> MGALRIDSHQHFWRYRAADYPWIGAGMGVLARDYLPDALHPLMHAQALGASIAVQARAGRDETAFLLELACDEARIAAVVGWEDLRAPQLAERVAEWRGTKLRGFRHQLQDEADVRAFVDDADFARGVAWLQANDYVYDVLVFERQLPDVQAFCARHDAHWLVLDHAGKPALAEFDRDDTAL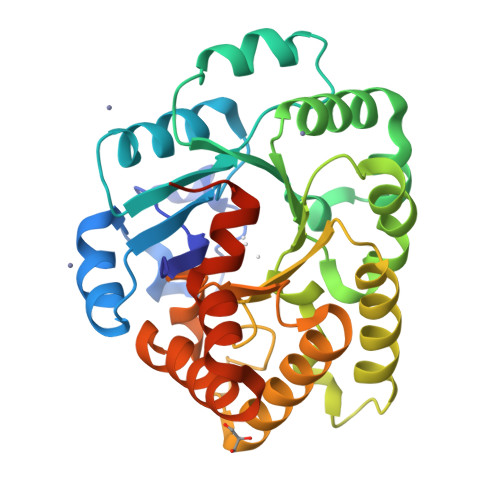ARWRAALRELAALPHVVCKLSGLVTEADWRRGLRASDLRHIEQCLDAALDAFGPQRLMFGSDWPVCLLAASYDEVASLVERWAESRLSAAERSALWGGTAARCYALPEPADARLAENLYFQ> MANFLTKNFVWILAAGVGVWFYQKADNAAKTATKPIADFLAELQ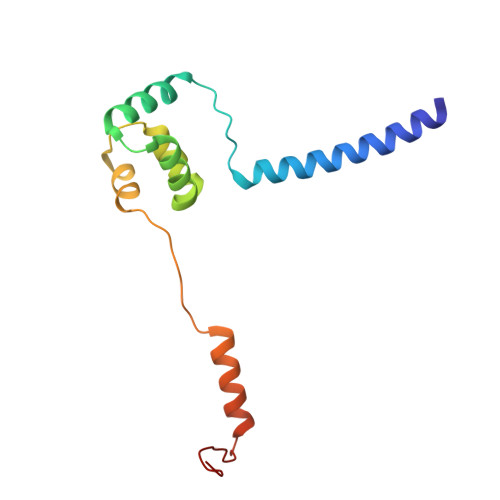FLVNGSNYVKFPNAGFVLTRDALQDDFIAYDDRIKAWLGTHDRHKDFLAEILDHERRVKPVYRKLIGNIIDASTIRAASGVEL>[2x]SELRKLFYSADAVCFDVDSTVIREEGIDELAKICGVEDAVSEMTRRA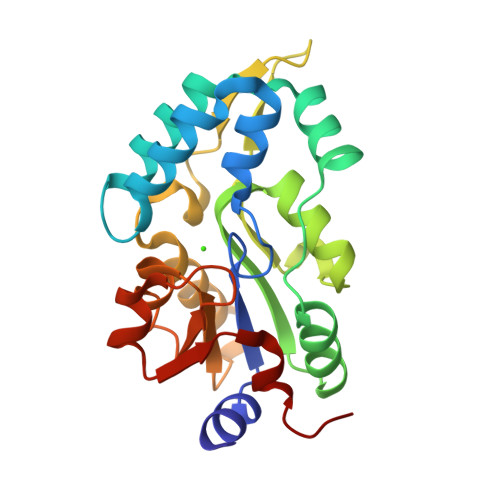MGGAVPFKAALTERLALIQPSREQVQRLIAEQPPHLTPGIRELVSRLQERNVQVFLISGGFRSIVEHVASKLNIPATNVFANRLKFYFNGEYAGFDETQPTAESGGKGKVIKLLKEKFHFKKIIMIGDGATDMEACPPADAFIGFGGNVIRQQVKDNAKWYITDFVELLGELE>MFAFYFLTACISLKGVFGVSPSYNGLGLTPQMGWDNWNTFACDVSEQLLLDTADRISDLGLKDMGYKYIILDDCWSSGRDSDGFLVADEQKFPNGMGHVADHLHNNSFLFGMYSSAGEYTCAGYPGSLGREEEDAQFFANNRVDYLKYANCYNKGQFGTPEISYHRYKAMSDALNKTGRPVFYSLCNWGQDLTFYWGSGIANSWRMSGDVTAEFTRPDSRCPCDGDEYDCKYAGFHCSIMNILNKAAPMGQNAGVGGWNDLDNLEVGVGNLTDDEEKAHFSMWAMVKSPLIIGANVNNLKASSYSIYSQASVIAINQDSNGIPATRVWRYYVSDTDEYGQGEIQMWSGPLDNGDQVVALLNGG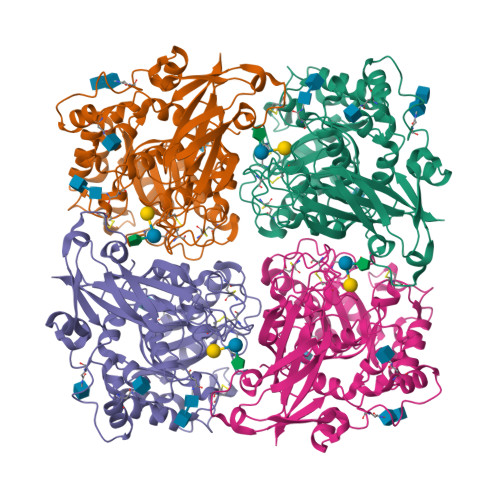SVSRPMNTTLEEIFFDSNLGSKKLTSTWDIYDLWANRVDNSTASAILGRNKTATGILYNATEQSYKDGLSKNDTRLFGQKIGSLSPNAILNTTVPAHGIAFYRLRPSSDYKDDDDK[4x]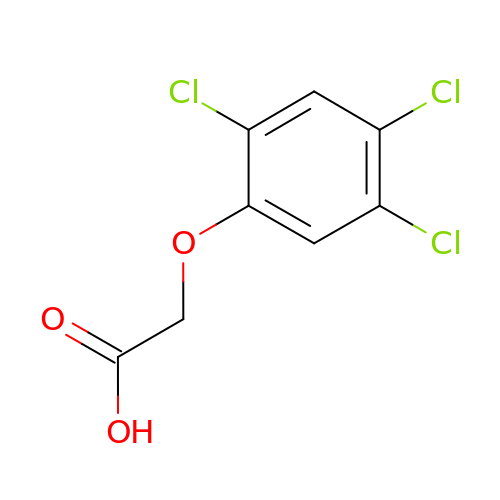2-[2,4,5-tris(chloranyl)phenoxy]ethanoic acid | C8 H5 Cl3 O3 | SMYMJHWAQXWPDB-UHFFFAOYSA-N> YPMNINDALTSILASKKYRALCPDTVRRILTEEWGRHKSPKQTVEAARTRLHGICGAYVTPESLKAAAAALSAGDVKKALSLHASTKERLAELDTLYDFIFSAE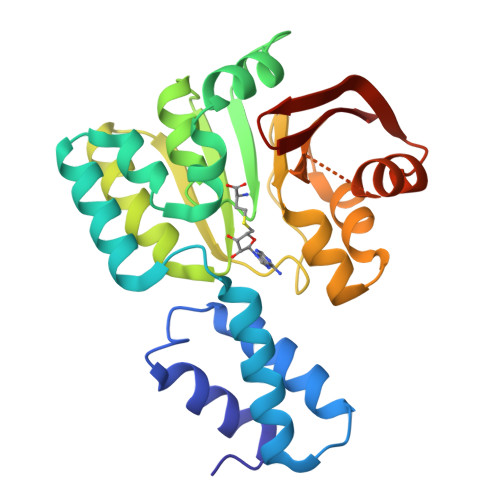TPRRVLDIACGLNPLALYERGIASVWGCDIHQGLGDVITPFAREKDWDFTFALQDVLCAPPAEAGDLALIFKLLPLLEREQAGSAMALLQSLNTPRMAVSFPTRSLGGRGKGMEANYAAWFEGGLPAEFEIEDKKTIGTELIYLIKKNG N-(3-fluorophenyl)-5-methyl-1,3,4-thiadiazol-2-amine 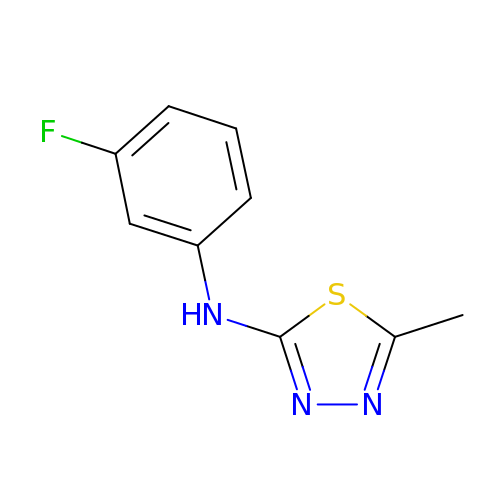| C9 H8 F N3 S | YJCLSQDDYPKKDX-UHFFFAOYSA-N>[4x]MEGPIPPHSLEAEQSVLGSILLDSDVMDEVEGLLPSPEAFYAEAHRKIYAAMQALRSQGRPVDLVTLSEELSRRGQLEEVGGTAYLLQLSEATPTAAYAEHYARIVAEKWTLRRLIQAAGEAMRLAYEEAGSLDEILDTAGKKILEVALTKTDTEARPMRELVHETFEHIEALFQNKGEVAGVRTGFK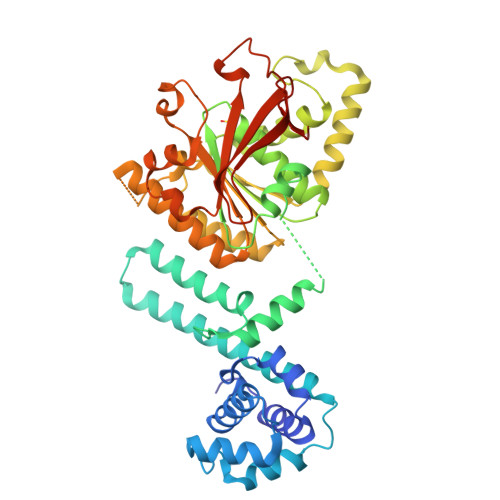ELDQLIGTLGPGSLNIIAARPAMGKTAFALTIAQNAALKEGVGVGIYSLEMPAAQLTLRMMCSEARIDMNRVRLGQLTDRDFSRLVDVASRLSEAPIYIDDTPDLTLMEVRARARRLVSQNQVGLIIIDYLQLMSGPGSGKSGENRQQEIAAISRGLKALARELGIPIIALSQLSRAVEARPNKRPMLSDLRESGSIEQDADLVMFIYRDEYYNPHSEKAGIAEIIVGKQRNGPTGTVELQFHASHVRFNDLARDA> KRKDITLLNPIVRKFQYGQHTVTLETGMMARQATAAVMVSMDDTAVFVTVVGQKKAKPGQDFFPLTVNYQERTYAAGRIPGSFFRREGRPSEGETLIARLIDRPIRPLFPEGFVNEVQVIATVVSVNPQVNPDIVAMIGASAALSLSGIPFNGPIGAARVGYINDQYVLNPTQDELKESKLDLVVAGTEAAVLMVESEAQLLSEDQMLGAVVFGHEQQQVVIQNINELVKEAGKPRWDWQPEPVNEALNARVAALAEARLSDAYRITDKQERYAQVDVIKSETIATLLAEDETLDENELGEILHAIEKNVVRSRVLAGEPRIDGREKD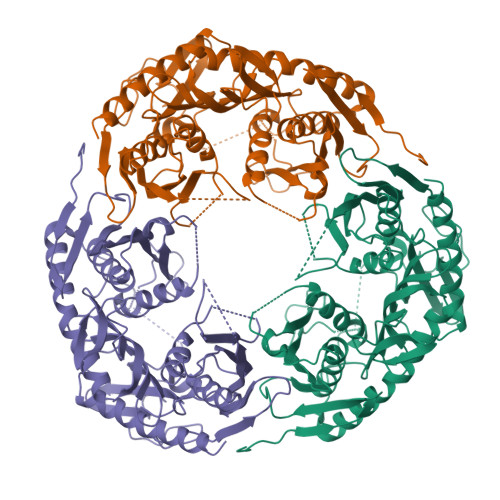MIRGLDVRTGVLPRTHGSALFTRGETQALVTATLGTARDAQVLDELMGERTDTFLFHYNFPPYSVGETGMVGSPKRREIGHGRLAKRGVLAVMPDMDKFPYTVRVVSEITESNGSSSMASVCGASLALMDAGVPIKAAVAGIAMGLVKEGDNYVVLSDILGDEDHLGDMDFKVAGSRDGISALQMDIKIEGITKEIMQVALNQAKGARLHILGVMEQAINAPRGDHHHHHH> GAMGYKDNIRHGVCWIYYPDGGSLVGEVNEDGEMTGEKIAYVYPDERTALYGKFIDGEMIEGKLATLMSTEEGRPHFELMPGNSVYHFDKSTSSCISTNALLPDPYESERVYVAESLISSAGEGLFSKVAVGPNTVMSFANGVRITHQEVDSRDWALNGNTLSLDEETVIDVPEPYNHVSKYCASLGHKANHSFTPNCIYDMFVHPR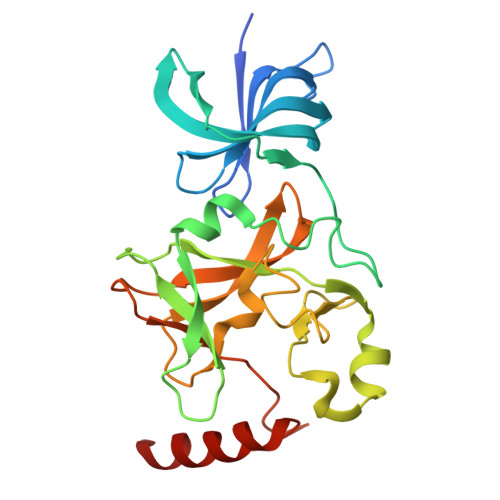FGPIKCIRTLRAVEADEELTVAYGYDHSPPGKSGPEAPEWYQVELKAFQATQQK> GPLGSVEEIRLPRAGGPLGLSIVGGSDHSSHPFGVQEP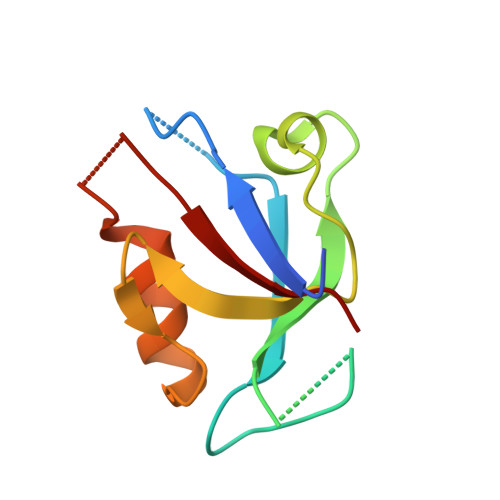GVFISKVLPRGLAARSGLRVGDRILAVNGQDVRDATHQEAVSALLRPCLELSLLVRRD>MLNTTFANAKFANPFMNASGVHCMTIEDLEELKASQAGAYITKSSTLEKREGNPLPRYVDLELGSINSMGLPNLGFDYYLDYVLKNQKENAQEGPIFFSIAGMSAAEN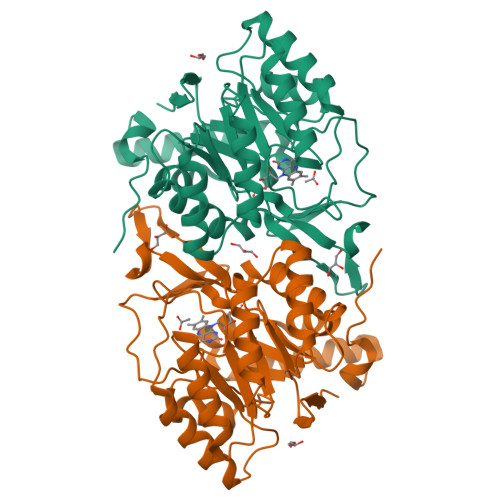IAMLKKIQESDFSGITELNLSCPNVPGKPQLAYDFEATEKLLKEVFTFFTKPLGVKLPPYFDLVHFDIMAEILNQFPLTYVNSVNSIGNGLFIDPEAESVVIKPKDGFGGIGGAYIKPTALANVRAFYTRLKPEIQIIGTGGIETGQDAFEHLLCGATMLQIGTALHKEGPAIFDRIIKELEEIMNQKGYQSIADFHGKLKSL[2x]2-(3-methylphenyl)-N-(pyridin-3-yl)acetamide 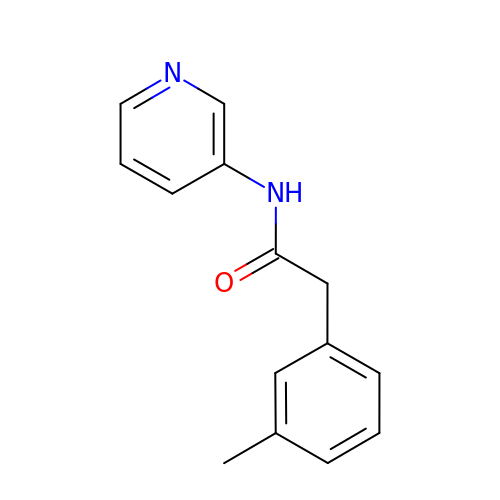| C14 H14 N2 O | AHPALPGTXJXWGY-UHFFFAOYSA-N(1S,2S)-2-cyano-N-[(1S,5R)-3-(5-fluoro-2-{[1-(2-hydroxyethyl)-1H-pyrazol-4-yl]amino}pyrimidin-4-yl)-3-azabicyclo[3.1.0]hexan-1-yl]cyclopropane-1-carboxamide | C19 H21 F N8 O2 | 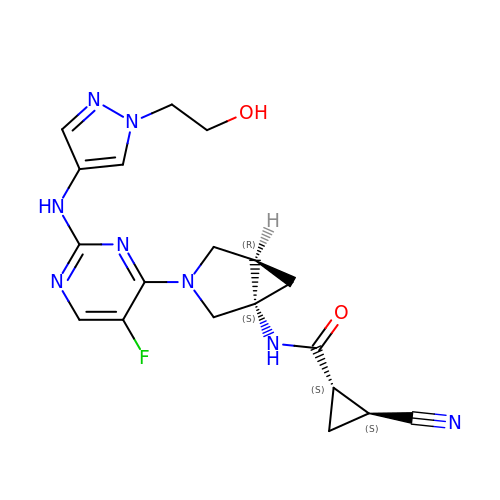OCNRQCROIYCWQL-NTHKCUKCSA-N> MTFRKSFDCYDFYDRAKVGEKCTQDDWDLMKIPMKAMELKQKYGLDFKGEFIPTDKDMMEKLFKAGFEMLLECGIYCTDTHRIVKYTEDEIWDAINNVQKEFVLGTGRDAVNVRKRSVGDKAKPIVQGGPTGSPISEDVFMPVHMSYALEKEVDTIVNGVMTSVRGKSPIPKSPYEVLAAKTETRLIKNACAMAGRPGMGVOGPETSLSAQGNISADCTGGMTCTDSHEVSQLNELKIDLDAISVIAHYKGNSDIIMDEQMPIFGGYAGGIEETTIVDVATHINAVLMSSASWHLDGPVHIRWGSTNTRETLMIAGWACATISEFTDILSGNQYYPCAGPCTEMCLLEASAQSITDTASGREILSGVASAKGVVTDKTTGMEARMMGEVAR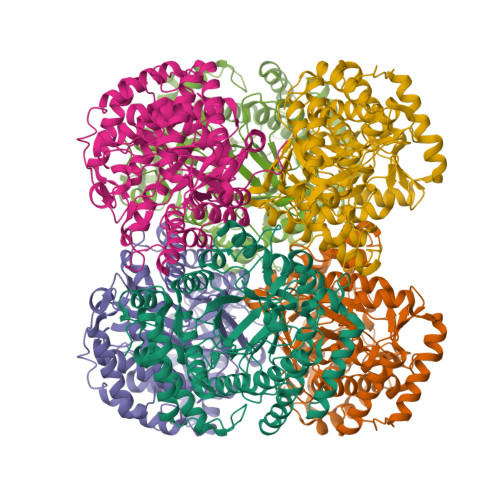ATAGVEISEVNVILDKLVSLYEKNYASAPAGKTFQECYDVKTVTPTEEYMQVYDGARKKLEDLGLVF>AVSDTSGQTLNEHNELEVRYSEVLRELERRIIHLQRRINMQLQQLTLLQHNIKTQVSQILRVEVDIDVALRACKGSCARYLEYRLDKEKNLQLEKAASYIANLKFERFEEVVVEETLNR[4x];>SSTHVNAQKEIENRYKEVKIRIESTVAGSLRSMKSVLEHLRAKMQRMEEAIKTQKELCSAPCTVNCRVPVVSGMHCEDIYRNGGRTSEAYYIQPDLFSEPYKVFCDMESHGGGWTVVQNRVDGSS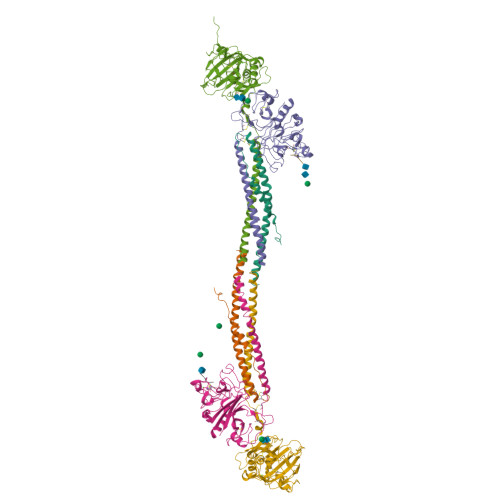NFARDWNTYKAEFGNIAFGNGKSICNIPGEYWLGTKTVHQLTKQHTQQVLFDMSDWEGSSVYAQYASFRPENEAQGYRLWVEDYSGNAGNALLEGATQLMGDNRTMTIHNGMQFSTFDRDNDNWNPGDPTKHCSREDAGGWWYNRCHAANPNGRYYWGGIYTKEQADYGTDDGVVWMNWKGSWYSMRQMAMKLRPKWP[4x];>[4x]DSGQKTVQKILEEVRILEQIGVSHDAQIQELSEMWRVNQQFVTRLQQQLVDIRQTCSRPCQDTTANKISPITGKDCQQVVDNGGKDSGLYYIKPLKAKQPFLVFCEIENGNGWTVIQHRHDGSVNFTRDWVSYREGFGYLAPTLTTEFWLGNEKIHLLTGQQAYRLRIDLTDWENTHRYADYGHFKLTPESDEYRLFYSMYLDGDAGNAFDGFDFGDDPQDKFYTTHLGMLFSTPERDNDKYEGSCAEQDGSGWWMNRCHAGHLNGKYYFGGNYRKTDVEFPYDDGIIWATWHDRWYSLKMTTMKLLPMGRDLSGHGGQQQSK;>GHRPX[4x]(3R,4R)-1-(2,2-DIFLUORO-ETHYL)-PYRROLIDINE-3,4-DICARBOXYLIC ACID 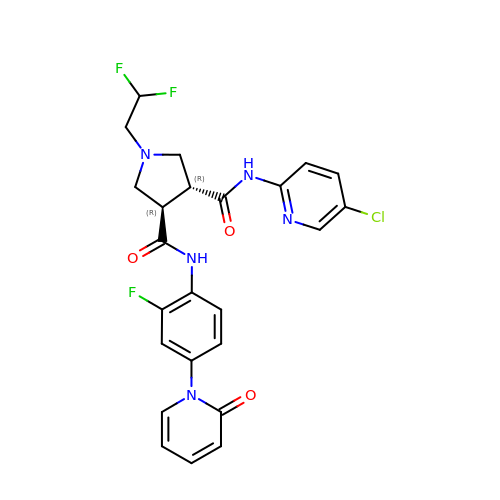3-[(5-CHLORO-PYRIDIN-2-YL)-AMIDE]-4-{[2-FLUORO-4-(2-OXO-2H-PYRIDIN-1-YL)-PHENYL]-AMIDE} | C24 H21 Cl F3 N5 O3 | DVMCMTVFXINJGW-IRXDYDNUSA-N>[2x]MAHHHHHHMANYSTNDFKPGLKVMLDSNPCSIMENEYVKPGKGQAFNRVKLRNLKTGKVLEKTFKSGDTLEAADIVEVEMNYLY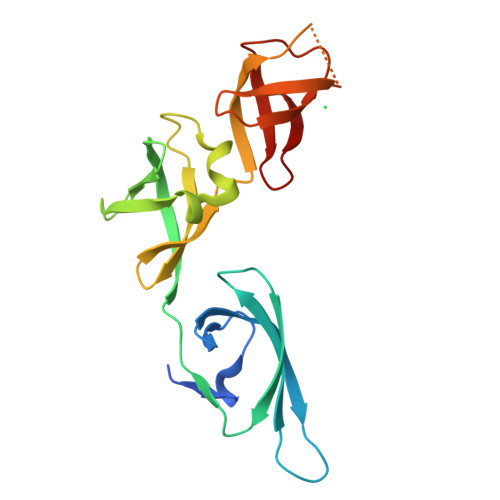NDGEMWHFMDPESFEQIAADKTAMGDAAKWLKDDSNETCTIMLFNGVPLNVNAPNFVVLKVVETDPGVRGDTSGGGGKPAKLETGAVVRVPLFVQQEESVRVDTRTGEYLERA>[4x]MTLQEQIMKALHVQPVIDPKAEIRKRVDFLKDYVKKTGAKGFVLGI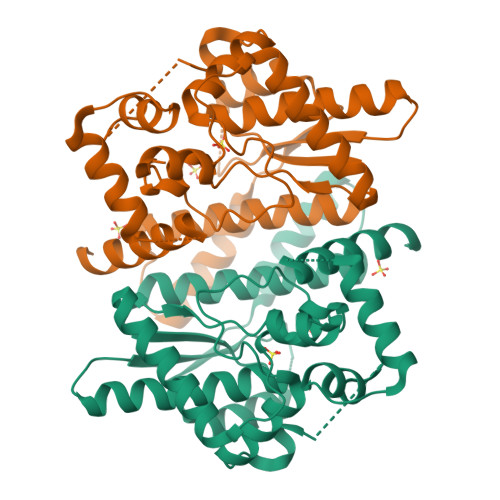SGGQDSTLAGRLAQLAVEEIRNEGGNATFIAVRLPYKVQKDEDDAQLALQFIQADQSVAFDIASTVDAFSNQYENLLDESLTDFNKGNVKARIRMVTQYAIGGQKGLLVIGTDHAAEAVTGFFTKFGDGGADLLPLTGLTKRQGRALLQELGADERLYLKMPTADLLDEKPGQADETELGITYDQLDDYLEGKTVPADVAEKIEKRYTVSEHKRQVPASMFDDWWKLAAALEHHHHHH Phosphopantetheinyl transferases (PPTases) are essential enzymes involved in primary and secondary metabolite biosynthetic pathways. They catalyze the transfer of the 4ʹ‐phosphopantetheinyl (Ppant) moiety of coenzyme A (CoA) to a strictly conserved serine residue of carrier protein (CP) domains present in fatty acid synthases (FASs), polyketide synthases (PKSs) and non-ribosomal peptide synthetases (NRPSs). The covalent attachment of the 20 Å-long Ppant arm to CP domains allows tethering substrates and chemical intermediates through a reactive thioester bond and transferring them to the different catalytic centers of the synthases where enzymatic modifications can proceed. Owing to their role in activating enzymes essential for bacterial viability and pathogenicity, phosphopantetheinyl transferases represent novel and attractive drug targets.

P. aeruginosa has a unique PPTase, PcpS, which was shown to be essential for the growth of the bacteria. In the course of this study, we also resolved the crystal structure of PcpS in the presence of CoA at 2.40 Å resolution. PcpS crystallizes in space group P1 with four molecules in the asymmetric unit. Thus, the crystal structure confirms that PcpS is a monomeric Sfp-like PPTase (Sfp: surfactin phosphopantetheinyl transferase from Bacillus subtilis). Despite low sequence identity, PcpS shares a high degree of structural conservation with the mycobacterial PPTases. The cofactor in PcpS occupies the same position and configuration as those found for CoA in the PptAb structure with the Ppant arm perfectly visible in electron density. The Lys72 → Val90 substitution induces the loss of a hydrogen bond with CoA, which is more than compensated by the change of Gly76 in PptAb to Arg94 in PcpS. Tight binding of CoA to PcpS is completed by hydrogen bonds between Glu175, probably the PcpS catalytic base, to another oxygen of the β-phosphate and to the nitrogen atom of the β-alanine. Despite several attempts, either by co-crystallization or by soaking, no structure of a complex between PcpS and 8918 could be obtained. Indeed, Arg94 in PcpS, found at the same position as Gly76 in PptAb, a residue that takes part to the CoA-binding site, would cause a steric clash with the diethylphenyl group of the inhibitor.

>[4x]GSHMRAMNDRLPSFCTPLDDRWPLPVALPGVQLRSTRFDPALLQPGDFALAGIQPPANILRAVAKRQAEFLAGRLCARAALFALDGRAQTPAVGEDRAPVWPAAISGSITHGDRWAAALVAARGDWRGLGLDVETLLEAERARYLHGEILTEGERLRFADDLERRTGLLVTLAFSLKESLFKALYPLVGKRFYFEHAELLEWRADGQARLRLLTDLSPEWRHGSELDAQFAVLDGRLLSLVAVGA N-(CYCLOPROPYLMETHYL)-4-(METHYLOXY)-3-({5-[3-(3-PYRIDINYL)PHENYL]-1,3-OXAZOL-2-YL}AMINO)BENZENESULFONAMIDE 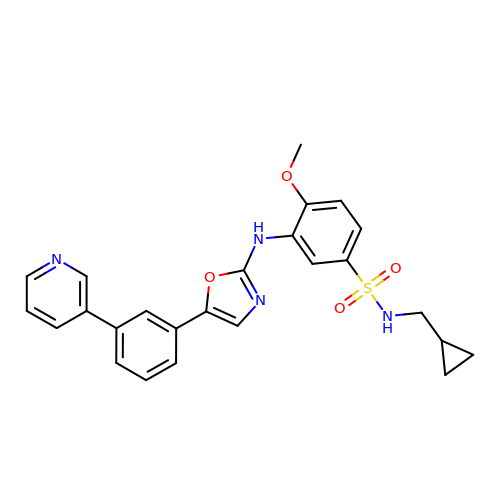| C25 H24 N4 O4 S | KRGKAARWVPUWSY-UHFFFAOYSA-N>GSHMEAVQNRIVEAAERVPGVRGVIHLRARYVGQDIAADMIIGVDPENTVEQAHEICEAVQAAVCGKIRRIESLHVSAEAREIGDTTKPSF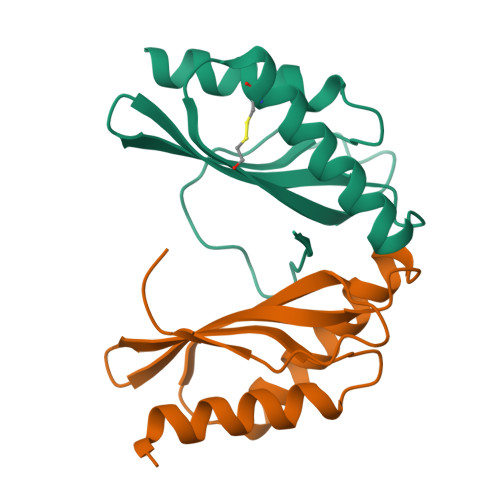SDQPLSFDEVMLSKVDN[2x]> MVKLSSDINLRDFGNNEYLSSVQDEAIRFATEQTDEILSLYSQHADTEGGRYVCADTFKELFPAFENKEDRATVNNAIHNSAAVLSSTQFDEVLKRDEPQKKEVIFVTGIPGSGKTSTVKNMMMQDTTKLLFEGQLARPQSAFRKIEQCLERNLEVTIVAVSMRAERASDNTYKRFNEYGRGASIGIMADIQANLPDGLKQIRDKFGDAVKIVGINQDRNSEFIDKFDDVIKMLSLGSQEQILGRLAEKIQSDFDSGKISRECFNQAKGSMDLESVFAKKEYSQQRVVTNSKGVTLETKSANELWSKVEQIPVTGMKAGIYLLGQAKKAETGQTYSGEIIYKDAAAVFQKTKNGLVRHNATHNEERLAKLVEIGQNVSIGS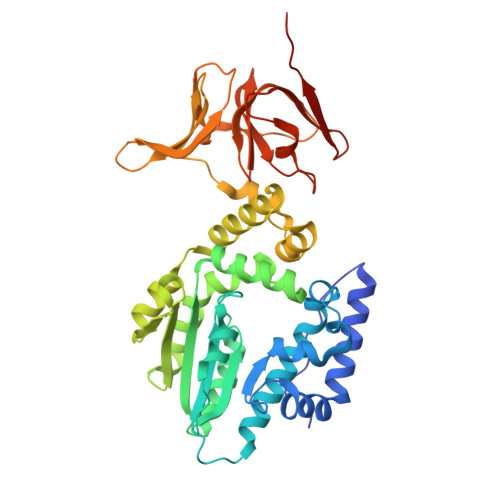NKGKLIVKSLEYSAKKSISR>MGSSHHHHHHENLYFQSMASMKTELIRTISLYDTIILHRHVRPD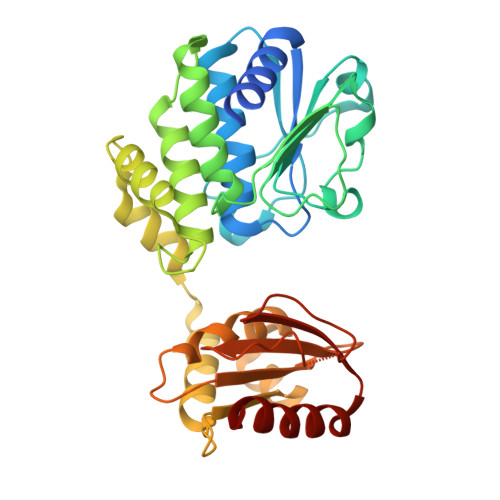PDAYGSQCGLTEILRETYPEKNIFAVGTPEPSLSFLYSLDEVDNETYEGALVIVCDTANQERIDDQRYPSGAKLMKIDHHPNEDPYGDLLWVDTSASSVSEMIYELYLEGKEHGWKLNTKAAELIYAGIVGDTGRFLFPNTTEKTLKYAGELIQYPFSSSELFNQLYETKLNVVKLNGFIFQNVSLSENGAASVFIKKDTLEKFGTTASEASQLVGTLGNISGIRAWVFFVEEDDQIRVRFRSKGPVINGLARKYNGGGHPLASGASIYSWDEADRILADLETLCKEHE[4x]>GAMGYIDQQ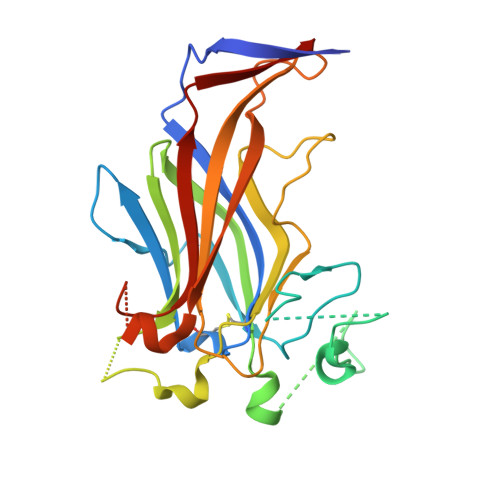YVVDSQVRDTVQINMDIYVNTKCDWLQINVRDQTMDRKLVLEELQLEEMPFFIPYDTKVNDINEIITPELDEILGEAIPAEFREKLDTRSFFDESDPNKAHLPEFNGCHVFGSIPVNRVSGELQITAKSLGYVASRKAPLEELKFNHVINEFSFGDFYPYIDNPLDNTAQFNQDEPLTTYVYYTSVVPTLFKKLGAEVDTNQYSVNDYRYLYKDVAAKGDKMPGIFFKYNFEPLSIVVSDVRL[2x]> EEEEE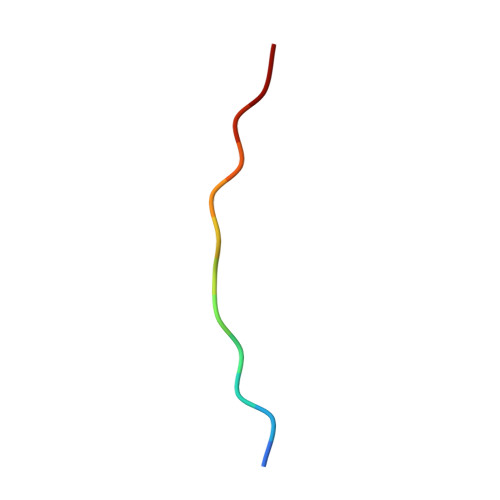EEEEEEE> MKNCVIVSAVRTAIGSFNGSLASTSAIDLGATVIKAAIERAKIDSQHVDEVIMGNVLQAGLGQNPARQALLKSGLAETVCGFTVNKVCGSGLKSVALAAQAIQAGQAQSIVAGGMENMSLAPYLLDAKARSGYRLGDGQVYDVILRDGLMCATHGYHMGITAENVAKEYGITREMQDELALHSQRKAAAAIESGAFTAEI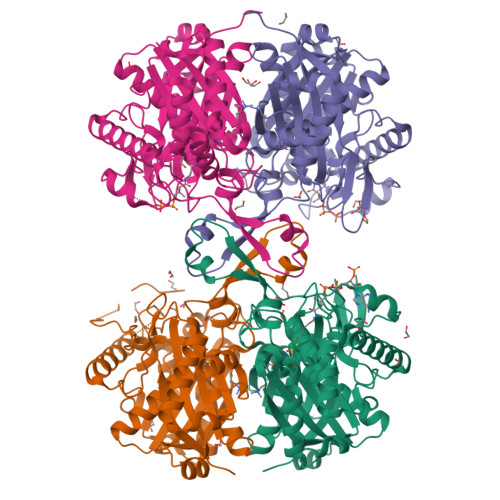VPVNVVTRKKTFVFSQDEFPKANSTAEALGALRPAFDKAGTVTAGNASGINDGAAALVIMEESAALAAGLTPLARIKSYASGGVPPALMGMGPVPATQKALQLAGLQLADIDLIEANEAFAAQFLAVGKNLGFDSEKVNVNGGAIALGHPIGASGARILVTLLHAMQARDKTLGLATLCIGGGQGIAMVIERLN;> MKNCVIVSAVRTAIGSFNGSLASTSAIDLGATVIKAAIERAKIDSQHVDEVIMGNVLQAGLGQNPARQALLKSGLAETVCGFTVNKVCGSGLKSVALAAQAIQAGQAQSIVAGGMENMSLAPYLLDAKARSGYRLGDGQVYDVILRDGLMCATHGYHMGITAENVAKEYGITREMQDELALHSQRKAAAAIESGAFTAEIVPVNVVTRKKTFVFSQDEFPKANSTAEALGALRPAFDKAGTVTAGNASGINDGAAALVIMEESAALAAGLTPLARIKSYASGGVPPALMGMGPVPATQKALQLAGLQLADIDLIEANEAFAAQFLAVGKNLGFDSEKVNVNGGAIALGHPIGASGARILVTLLHAMQARDKTLGLATLCIGGGQGIAMVIERL;> ASMKNCVIVSAVRTAIGSFNGSLASTSAIDLGATVIKAAIERAKIDSQHVDEVIMGNVLQAGLGQNPARQALLKSGLAETVCGFTVNKVCGSGLKSVALAAQAIQAGQAQSIVAGGMENMSLAPYLLDAKARSGYRLGDGQVYDVILRDGLMCATHGYHMGITAENVAKEYGITREMQDELALHSQRKAAAAIESGAFTAEIVPVNVVTRKKTFVFSQDEFPKANSTAEALGALRPAFDKAGTVTAGNASGINDGAAALVIMEESAALAAGLTPLARIKSYASGGVPPALMGMGPVPATQKALQLAGLQLADIDLIEANEAFAAQFLAVGKNLGFDSEKVNVNGGAIALGHPIGASGARILVTLLHAMQARDKTLGLATLCIGGGQGIAMVIERL;> ASMKNCVIVSAVRTAIGSFNGSLASTSAIDLGATVIKAAIERAKIDSQHVDEVIMGNVLQAGLGQNPARQALLKSGLAETVCGFTVNKVCGSGLKSVALAAQAIQAGQAQSIVAGGMENMSLAPYLLDAKARSGYRLGDGQVYDVILRDGLMCATHGYHMGITAENVAKEYGITREMQDELALHSQRKAAAAIESGAFTAEIVPVNVVTRKKTFVFSQDEFPKANSTAEALGALRPAFDKAGTVTAGNASGINDGAAALVIMEESAALAAGLTPLARIKSYASGGVPPALMGMGPVPATQKALQLAGLQLADIDLIEANEAFAAQFLAVGKNLGFDSEKVNVNGGAIALGHPIGASGARILVTLLHAMQARDKTLGLATLCIGGGQGIAMVIER(2E,4E,6Z,8E)-8-{3-[(2S)-butan-2-yl]-2-(3-methylbutyl)cyclohex-2-en-1-ylidene}-3,7-dimethylocta-2,4,6-trienoic 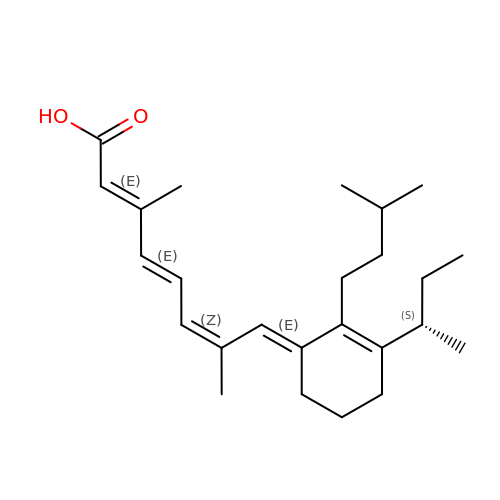acid | C25 H38 O2 | USDOYFQDHIMGBQ-CKASWENUSA-N> QYSPNTQQGRTSIVHLFEWRWVDIALECERYLAPKGFGGVQVSPPNENVAIYNPFRPWWERYQPVSYKLCTRSGNEDEFRNMVTRCNNVGVRIYVDAVINHMCGNAVSAGTSSTCGSYFNPGSRDFPAVPYSGWDFNDGKCKTGSGDIENYNDATQVRDCRLTGLLDLALEKDYVRSKIAEYMNHLIDIGVAGFALDASKHMWPGDIKAILDKLHNLNSNWFPAGSKPFIYQEVIDLGGEPIKSSDYFGNGRVTEFKYGAKLGTVIRKWNGEKMSYLKNWGEGWGFVPSDRALVFVDNHDNQRGHGAGGASILTFWDARLYKMAVGFMLAHPYGFTRVMSSYRWPRQFQNGNDVNDWVGPPNNNGVIKEVTINPDTTCGNDWVCEHRWRQIRNMVIFRNVVDGQPFTNWYDNGSNQVAFGRGNRGFIVFNNDDWSFSLTLQ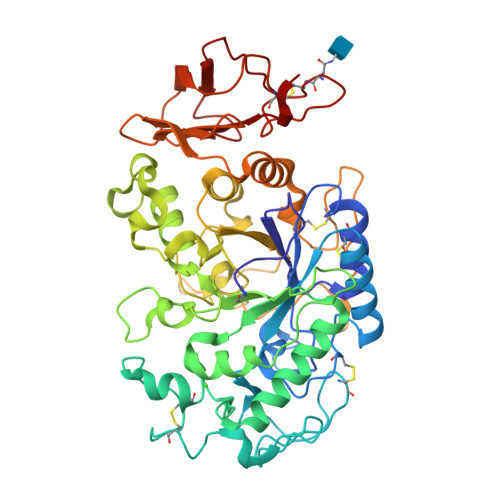TGLPAGTYCDVISGDKINGNCTGIKIYVSDDGKAHFSISNSAEDPFIAIHAESKL>[2x]YVEGQRKRRNTIHEFKKSAKTTLIKIDPALKIKTKKVNTADQCANRCTRNKGLPFTCKAFVFDKARKQCLWFPFNSMSSGVKKEFGHEFDLYENKDYIRNCIIGKGRSYKGTVSITKSGIKCQPWSSMIPHEHSFLPSSYRGKDLQENYCRNPRGEEGGPWCFTSNPEVRYEVCDIPQCSEVE

The growth/motility factor hepatocyte growth factor/scatter factor (HGF/SF) and its receptor, the tyrosine kinase MET, constitute a signalling system essential for embryogenesis and for tissue/organ regeneration in post-natal life. Two truncated forms of HGF/SF are produced by alternative splicing of the primary transcript: NK1 encodes the N domain and the first K domain (K1),16 while NK2 encodes the N, K1 and K2 domains. NK1 is a monomer in solution, but crystallises as a head-to-tail dimer and all available crystal structures of human and mouse NK1 yielded the same dimer. (c) The lysine-binding pocket of the kringle domain of NK1 is formed by a glycine loop at the top of pocket (E183 and G186), an aromatic “base” (W188) and sides (F162 and Y198), as well as a positively charged anchor at the bottom of the pocket (R197).

Ten out of the 24 validated hits had KD < 1 mM with MB605 being the best fragment hit with a KD value of 310 ± 40 μM. Only MB605 showed variation in chemical shifts for several NK1 residues, mainly in and around the lysine-binding pocket, for example E183, R181 and E184, yielding a KD of 110 μM ± 10 μM that compares well with the value obtained by SPR. MB605 consists of two parts, a furan and a propanoic acid moiety, resembling HEPES. A crystal structure of MB605 soaked into NK1 apo crystals (see ESI Tables S1 and S2† for crystallographic statistics) demonstrated a binding mode similar to HEPES in which the carboxylic acid group of MB605 forms two hydrogen bonds to R197 and one main-chain hydrogen bond to S161 through a water molecule. In comparison to HEPES, MB605 forms stronger polar interactions and hydrogen bonds to E183 via the furan ring, as well as additional polar interactions to R181. The furan ring packs tightly in the aromatic part of the pocket, stacking against W188 and resting perpendicular to Y198. In this orientation, MB605 is able to make π–π interaction to W188 and Y198. Additionally, one molecule of the cryoprotectant ethylene glycol is bound in the lysine-binding pocket, 3.5 Å away from the furan ring, and makes hydrogen bonds to G185 and G186, similar to the NK1_MES structure. MB605 on the other hand has its furan ring in an ideal orientation to form strong π–π interactions with both W188 and Y198, in addition to making stronger polar interactions and hydrogen bonds to E183 than any of the piperazine-like compounds and an additional polar interaction to R181; yielding the highest affinity reported here (KD = 310 μM). MB605 is a very small molecule (140 Da) but displays about ten times better affinity for NK1 than HEPES and can be grown towards the glycine loop gaining the chemical space occupied by the ethylene glycol molecule in the current crystal structure and enabling hydrogen bonding to the glycine loop with significant affinity gain.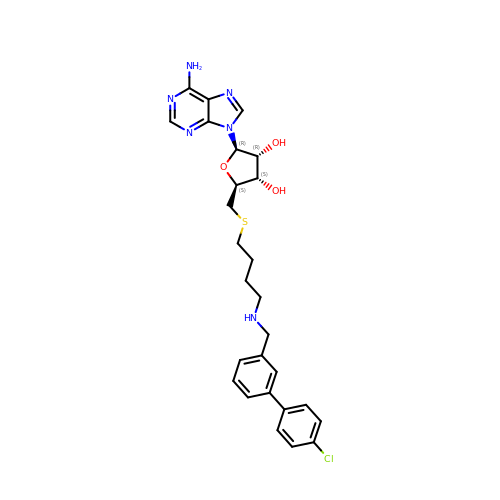5'-S-(4-{[(4'-chloro[1,1'-biphenyl]-3-yl)methyl]amino}butyl)-5'-thioadenosine | C27 H31 Cl N6 O3 S | UDFJXRJYAZANFF-VBHAUSMQSA-N> GPLGSATAPYNYSYIFKYIIIGDMGVGKSCLLHQFTEKKFMADCPHTIGVEFGTRIIEVSGQKIKLQ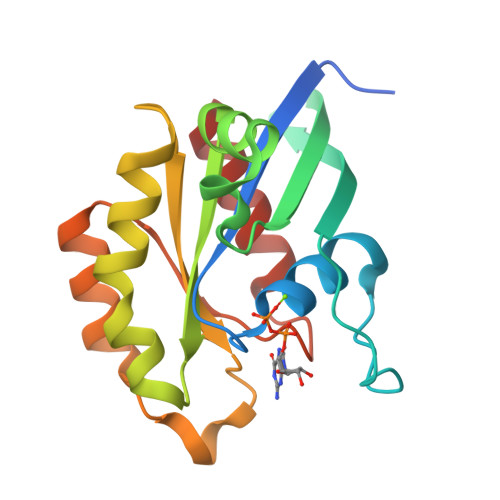IWDTAGQERFRAVTRSYYRGAAGALMVYDITRRSTYNHLSSWLTDARNLTNPNTVIILIGNKADLEAQRDVTYEEAKQFAEENGLLFLEASAKTGENVEDAFLEAAKKIYQN> GSHMSAPGPLVFTALSPDSLQLSWER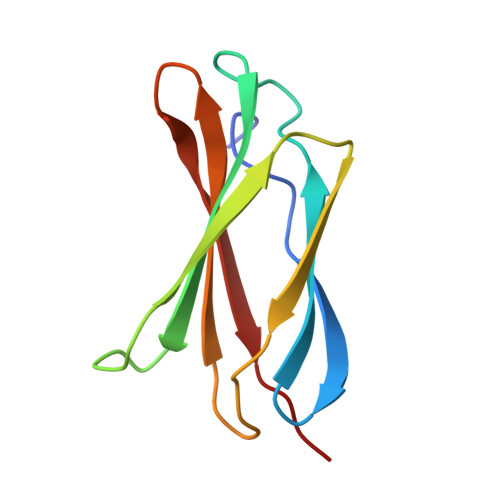PRRPNGDIVGYLVTCEMAQGGGPATAFRVDGDSPESRLTVPGLSENVPYKFKVQARTTEGFGPEREGIITIES> CGCGXAUUA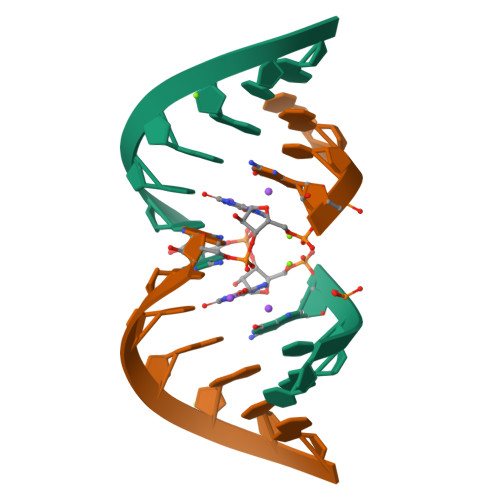GCG> YVYQLKDEVGEL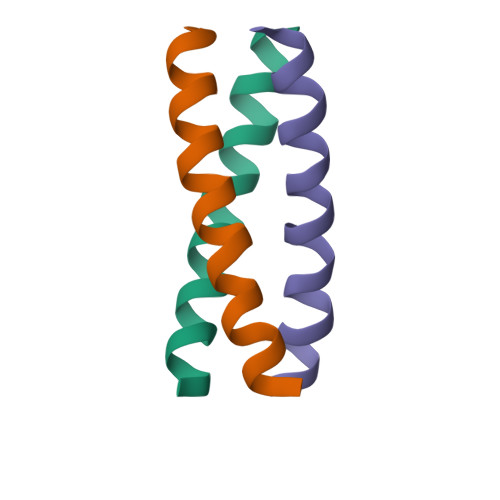KGEVRALKDEVKDLK>TRDQNGTWEMESNENFEGYMKALDIDFATRKIAVRLTQTLVIDQDGDNFKWKTTSTFRNYDVDF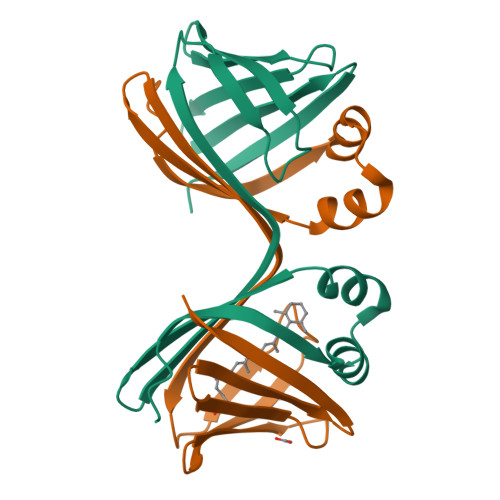TVGVEFDEYTKSLDNRHVKALVTWEGDVLVCVQKGEKENRGWKKWIEGDKLYLELTCGDQVCRQVFKKK[4x]> SHSTAETTLDSFFSRAGLVGEIDLPLEGTTNPNGYANWDIDITGYAQMRRKVELFTYMRFDAEFTFVACTPTGQVVPQLLQYMFVPPGAPKPDSRESLAWQTATNPSVFVKLSDPPAQVSVPFMSPASAYQWFYDGYPTFGEHKQEKDLEYGACPNNMMGTFSVRTVGTSKSKYPLVIRIYMRMKHVRAWIPRPMRNQNYLFKANPNYAGNFIKPTGASRTAITT;> LTIGNSTITTQEAANIIVGYGEWPSYCSDTRPDVSVNRFYTLDTKLWEKSSKGWYWKFPDVLTETGVFGQNAQFHYLYRSGFCIHVQCNASKFHQGALLVAVLPEYVIGTVAGGTGTEDSHPPYKQTQPGADGFELQHPYVLDAGIPISQLTVCPHQWINLRTNNCATIIVPYINALPFDSALNHCNFGLLVVPISPLDYDQGATPVIPITITLAPMCSEFAGLRQ;> GFPTELKPGTNQFLTTDDGVSAPILPNFHPTPCIHIPGEVRNLLELCQVETILEVNNVPTNATSLMERLRFPVSAQAGKGELCAVFRADPGRSGPWQSTLLGQLCGYYTQWSGSLEVTFMFT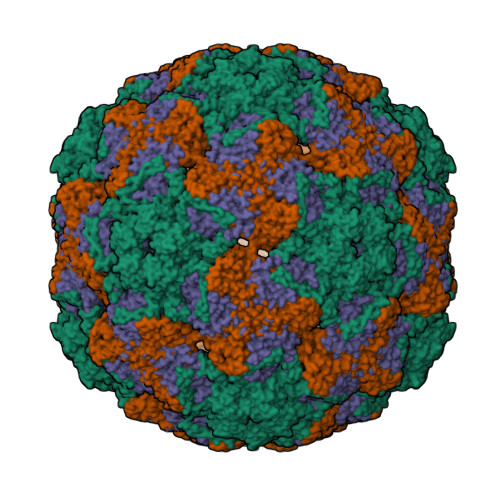GSFMATGKMLIAYTPPGGPLPKDRATAMLGTHVIWDFGLQSSVTLVIPTTGLVSIWYQTNYVVPIGAPNTAYIIALAAAQKNFTMQLCKDASDIL>SKVVYVSHDGTRRELDVADGVSLMQAAVSNGIYDIVGDCGGSASCATCHVYVNEAFTDKVPAANEREIGMLEGVT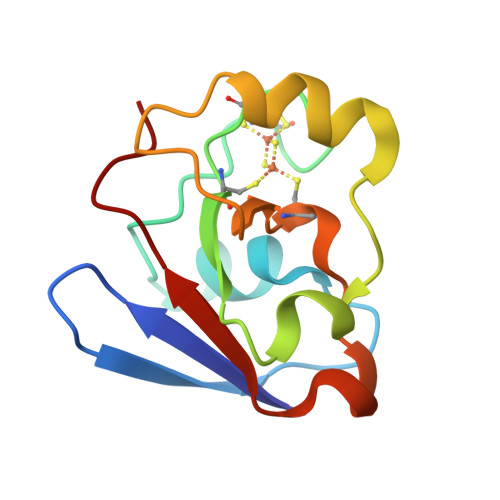AELKPNSRLCCQIIMTPELDGIVVDVPDRQW[3x]>MSFPYFISPEQAMRERSELARKGIARAKSVVALAYAGGVLFVAENPSRSLQKISELYDRVGFAAAGKFNEFDNLRRGGIQFADTRGYAYDRRDVTGRQLANVYAQTLGTIFTEQAKPYEVELCVAEVAHYGETKRPELYRITYDGSIADEPHFVVMGGTTEPIANALKESYAENASLTDALRIAVAALRAGSADTSGGDQPTLGVASLEVAVLDANRPRRAFRRITGSALQALLVDQESPQSDGESSG[14x];>[14x]TTIVALKYPGGVVMAGDRRSTQGNMISGRDVRKVYITDDYTATGIAGTAAVAVEFARLYAVELEHYEKLEGVPLTFAGKINRLAIMVRGNLAAAMQGLLALPLLAGYDIHASDPQSAGRIVSFDAAGGWNIEEEGYQAVGSGSLFAKSSMKKLYSQVTDGDSGLRVAVEALYDAADDDSATGGPDLVRGIFPTAVIIDADGAVDVPESRIAELARAIIESRSGADTFGSDGGEKHHHHHH;>[7x]MVIGLSTGSDDDDVEVIGGVDPRLIAVQ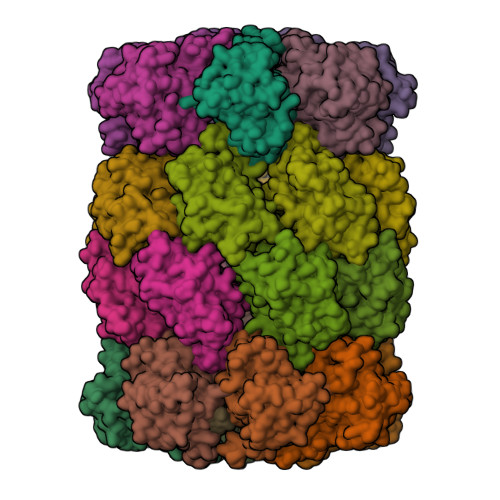ENDSDESSLTDLVEQPAKVMRIGTMIKQLLEEVRAAPLDEASRNRLRDIHATSIRELEDGLAPELREELDRLTLPFNEDAVPSDAELRIAQAQLVGWLEGLFHGIQTALFAQQMAARAQLQQMRQGALPPGVGKSGQHGHGTGQYL> GSMSTVRKITLKSSDGENFEIDEAVALESQTIKHMIEDDCTDNGIP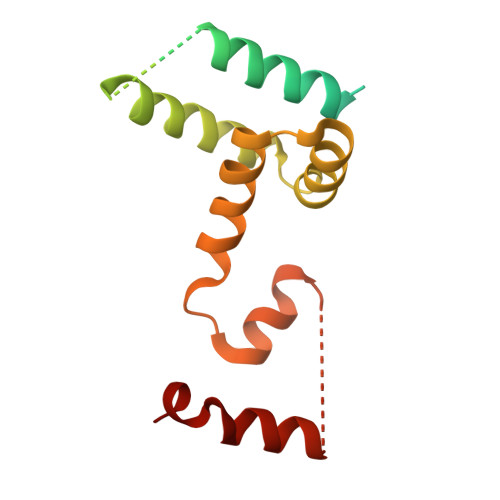LPNVTSKILSKVIEYCKRHVEAAEKSETTADAAAATTTTTVASGSSDEDLKTWDSEFIKVDQGTLFDLILAANYLNIKGLLDLTCQTVADMIKGKTPEEIRKTFNIKNDFTPEEEEEVRRENQWAFE>[2x]HAFRYSLNYPNIGHCIIINNKNFDRRTGMNPRNGTDVDAGNVMNVFRKLGYIVKVYNDQTVAQIMQVLTTVAHDDHSRCASLVCVLLSHGDE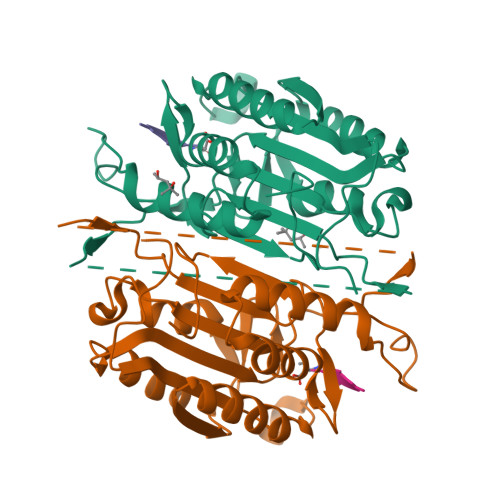GVFFGTDTSVDLKSLTSLFRGDRCPSLVGKPKLFFIQACRGTELDPGVETDHTDHPDIPDGRERIPVEADFLYAYSTVPGYYSWRNTMTGSWFIQSLCEMMTKYGSELELLQIMTRVNHKVALDFESTSNMPGFDAKKQIPCIVSMLTKEMYFTPSE>ASLNEKLKIEHAKKKRLFDLYINGSYEVSELDSM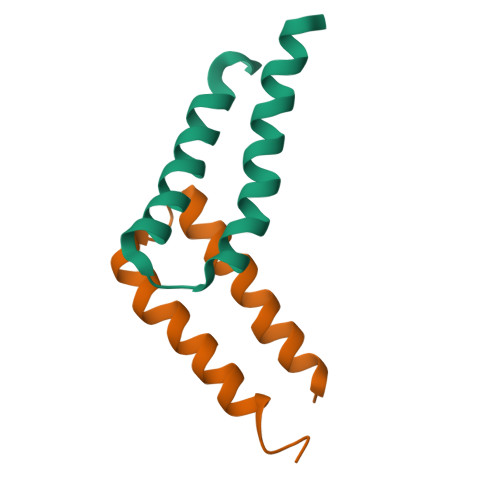MNDIDAQINYYEAQIEAN[8x]> GSMSSGLRAADFPRWKRHISEQ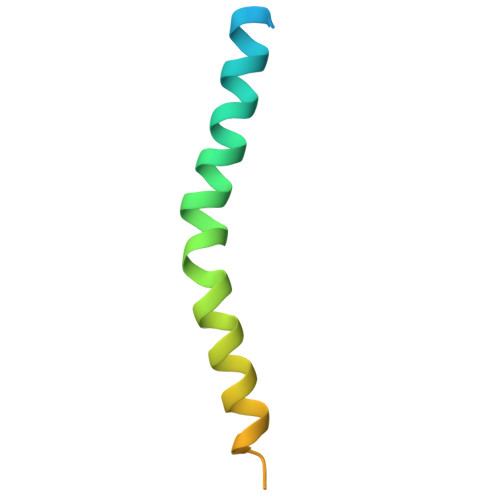LRRRDRLQRQAFEEIILQYNKLLEKSDLHSVLAQKLQAEKHDVPNRHEI We therefore set out to characterize two previously unstudied proteins from the shipworm symbiont Teredinibacter turnerae that were initially identified by the presence of carbohydrate binding domains appended to uncharacterized domains with probable redox functions. One of these was TERTU_3803, which contained both a CBM10 and a CBM2 domain attached to a range of distinct modules (via flexible linkers) that did not bare any sequence similarity with catalytic domains typically found within carbohydrate-active enzymes. Using a ‘module walking’ approach, we searched for other genes coding for these X-domains. This led to the identification of TERTU_2913, which lacks CBMs but contains predicted X122, X183 and X132 domains. Taken together, these sequence analyses suggested that TERTU_3803 and TERTU_2913 could have a role to play in cellulose metabolism, and furthermore that role is likely to be a redox one given the presence of cytochrome domains within their linear amino acid sequences.

In addition to our work on Ttpf08450-X173, we produced TtX122A and TtX122B, representing the X122 domains from TERTU_3803 and TERTU_2913, respectively. With the structure of TtX122A in hand, the structure of TtX122B could be solved to 2.2 Å via molecular replacement using a single protomer of TtX122A as an initial search model. Three molecules of TtX122B were present in the asymmetric unit, with chain B’s electron density most readily traced allowing modelling of residues 2 to 235 without breaks in the chain. Chains A and C had some areas that displayed more disorder, so there were breaks in the model between residues 190 and 192 in chain A and residues 162 and 165 in chain C. In addition to protein and water molecules, two magnesium ions were modelled into the electron density on each protomer in TtX122A based on coordination geometry and bond lengths [Fig. S4(a)]; these ions presumably bound from the crystallization medium. To check the oligomeric state of our TtX122 structures, PISA analysis was performed, which revealed that there were no significant molecular interfaces between protomers in the crystal for either structure, suggesting that the molecules would be expected to be monomeric in solution. Our subsequent structural analysis therefore focused on single protomers from each structure. The overall structures of TtX122A and TtX122B reveal that these domains adopt a β-jelly-roll fold [Figs. 4(a) and 4(b)]. Very similar results were observed for both TtX122A and TtX122B, in which there were only very small changes in antibody binding following X122 treatment in the case of some alginates (predominantly PAA and PAU) and wheat arabinoxylan, where twofold or threefold changes in antibody binding could be observed. We were unable to detect any fluorescence in the tissue from the X122A:GFP or X122B:GFP fusion protein alone and only a weak signal was observed for the CBM10-X122A:GFP protein.

>[3x]GSGFFVSDDFESSSVSQQPAGWDNFVGWQSNNPNNNSGQAVYAVVDNSRAYSGSQSVHFKGGAAPAQIVKALPQGLDRVYLKAMVYMSKKLGNEANDNHEHIMGVRANASGADNEIRFGQIKGHIGTNEVPSDDIAPPQSQWYSGPEITANDWHCVVVEMLAGDLAYHQLNAYVDGELLHSIDAANDWNNGGVNGNAHWLDGKFNYAFFGWHSFSNNDADVWMDDIEMSDAPLTCDGLEHHHHHH> MIEKVYCQEVKPELDGKKVRLAGWVYTNMRVGKKIFLWIRDSTGIVQAVVAKNVVGEETFEKAKKLGRESSVIVEGIVKADERAPGGAEVHVEKLEVIQAVSEFPIPENPEQASPELLLDYRHLHIRTPKASAIMKVKETLIMAAREW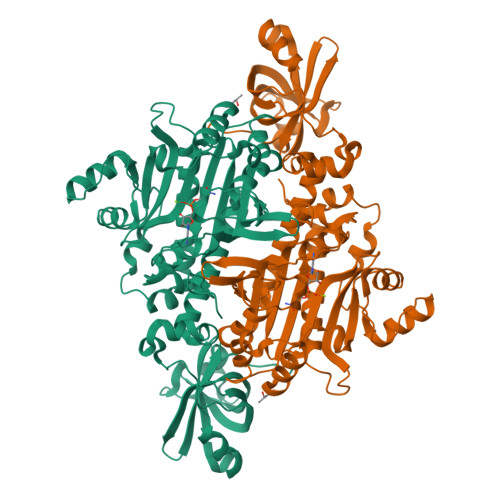LLKDGWHEVFPPILVTGAVEGGATLFKLKYFDKYAYLSQSAQLYLEAAIFGLEKVWSLTPSFRAEKSRTRRHLTEFWHLELEAAWMDLWDIMKVEEELVSYMVQRTLELRKKEIEMFRDDLTTLKNTEPPFPRISYDEAIDILQSKGVNVEWGDDLGADEERVLTEEFDRPFFVYGYPKHIKAFYMKEDPNDPRKVLASDMLAPEGYGEIIGGSQREDDYDKLLNRILEEGMDPKDYEWYLDLRRYGSVPHSGFGLGVERLVAWVLKLDHIRWAALFPRTPARLYP>[3x]QDDASDRQTREVLDPIVASLMEAQQIPGMAIALVRPEGTTISHYGAADRETGTPVDDDTLFEIGSLSKTLTATLASLAEVEGKLDFDAPVSRYLPELEGSAFDDISGLNLGTHTGGGLPLFVPDEVTDRASLMAWYREWQPTEPIGESRTYSNLGIGLLGLETAASLDGEFVPTMRAKVLAPLGMQDTWYDVPEARMADYAMGEDKDGQPTRVSPGVLDDEAYGIKTTAADLAKLVRANLHLADVDAELQQAIDATRQGHYRVGDMTQALIWEQYSLPVAPETLRAGQGYDMILEPNAAEALEPPQSPRDDVWVNKTGSTQGFGGYIVMLPGKHTGLVMLANKNYPNDARVEAAYRILSGLGAIDVP

To evaluate metal-ion affinity and to identify protein metal-binding sites for Sr2+ and Cs+, a class C β-lactamase (BLA) derived from the moderate halophile Chromohalobacter sp. 560 (HaBLA; molecular weight 39 536) was chosen as a model system. HaBLA, although a moderately halophilic periplasmic protein, has a particularly abundant content of acidic amino acids similar to those in extremely halophilic proteins. The crystal structure of a halophilic β-lactamase from Chromohalobacter sp. 560 (HaBLA) was determined to resolutions of between 1.8 and 2.9 Å in space group P31 using X-ray crystallography. Seven binding sites (site 1 to site 7) for divalent metal ions (Ca2+ and/or Sr2+) and one binding site (site 8) for Cs+ per HaBLA molecule were identified by X-ray diffraction studies including anomalous dispersion.

NQ-HaBLA was initially crystallized with Na+ and Ca2+ and the structure was determined to 1.8 Å resolution. The solvent content in the NQ-HaBLA crystal is 43.0%. The r.m.s.d. on Cα atoms between the monomers of WT-HaBLA and NQ-HaBLA are less than 0.5 Å; therefore, the N288Q/N321Q mutation did not significantly alter the overall structure of HaBLA. The crystallization of WT-HaBLA and NQ-HaBLA required divalent metal ions (Mg2+ or Ca2+). Both WT-HaBLA and NQ-HaBLA crystallized isomorphously, and both contained three HaBLA molecules in the asymmetric unit. The structural analysis of NQ-HaBLA shows that there are up to 11 locations for Ca2+ (Ca1–Ca11) in each asymmetric unit. The binding sites for Na+ were not identified in any of the measured HaBLA crystals because of its similar electron density to the O atom in water.> MLRSTGVSLYYRATAELDRLRGMLRGRARLERKVGLKRITFLMRTQTRYRVEQKAHWERAIVRKNVDSAAHEHGSGWQHLRNDLARQNLMLLPRTQQQLAQYEPLAFRAVMELCASRVAPPPPPMTAQVPEEAYATRPEDP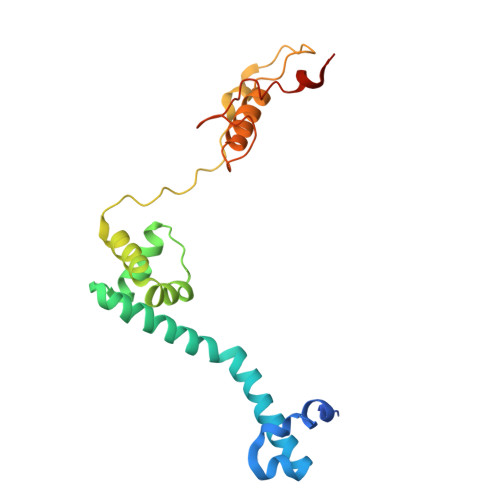KVAHPAARRQLEECVERMLCTGRSDVLQREGPRTTQAWMDAWKEYDLGSAAQK>[2x]MSLNITGIQSDWKVEKIEFAKLTGERARSAGANGRIGVHGKSCTVDIARITIDGQTGYGSSIHMTPEWAEDVIGRRL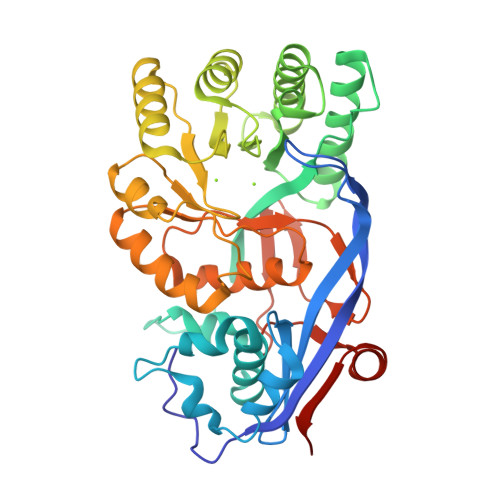LDLFDDRGRLREAYRLQLEYPVLDWLGQRQGKPVYDLVSGAHLETGASLVVPCYDTSLYFDDLHLADERAAVALMQEEAMQGYAKGQRHFKIKVGRGGRHMPLWEGTKRDIAIVRGISEVAGPAGKIMIDANNAYNLNLTKEVLAALSDVNLYWLEEAFHEDEALYEDLKEWLGQRGQNVLIADGEGLASPHLIEWATRGRVDVLQYDIIWPGFTHWMELGEKLDAHGLRSAPHCYGNAYGIYASGHLSAAVRNFEFVEYDDITIEGMDVSGYRIENGEIHVPATPGFGIVFDDELVTYLINRSGWSEGHHHHHH The basil EGS and petunia IGS are closely related to a number of other NADPH-dependent enzymes that act on phenylpropanoid-derived substrates. Structurally, the PIP-family proteins organize around an N-terminal, Rossman-fold domain, containing a core, six-stranded parallel β-sheet flanked on each face by an α-helical layer. In summary, a mechanistic scheme emerges in which binding of the coniferyl acetate substrate within the active site of EGS leads to deprotonation of the p-hydroxy group (PUSH) coupled with expulsion of acetate ion from the C1 substituent (PULL).

The monoclinic structure also contains two EGS/NADP+ complexes per asymmetric unit and was refined at 1.6-Å resolution resulting in crystallographic R-factors of 0.210 and 0.229. Intruigingly, in the monoclinic structure of unliganded EGS-NADP+, a nitrate anion from the crystallization medium occupies the site of the bridging water molecule, and may mimic the hydroxide ion that develops during the catalytic reaction. The structures of EGS complexed with NADP+ or NADPH provide the first structural characterization of nicotinamide-cofactor binding by the PIP family of enzymes (previous crystallographic analyses had yielded only apo-enzyme structures). The cofactor is bound through a large number of polar and non-polar interactions. The nicotinamide ring adopts the anti conformation with its B-face stacked against the side chain of Phe154 and its A-face directed towards the substrate-binding pocket. In contrast, the anti-conformer of the nicotinamide ring observed in EGS is consistent with the class-A reductase (donation of the pro-R hydride) activity of the PIP-family enzymes. Detailed inspection of the hydrogen-bonding network involving the ε-amino group of Lys132 suggests that this group exists formally in the unprotonated–NH2 state and is the donor in hydrogen-bond interactions with the 2′-hydroxyl group of the nicotinamide-ribose and the backbone carbonyl oxygen of residue 110. With an available lone pair of electrons, the amino group can serve as the acceptor in a hydrogen bond with the bridging water molecule, and most importantly, thereby act as a general base.

>MEENGMKSKILIFGGTGYIGNHMVKGSLKLGHPTYVFTRPNSSKTTLLDEFQSLGAIIVKGELDEHEKLVELMKKVDVVISALAFPQILDQFKILEAIKVAGNIKRFLPSDFGVEEDRINALPPFEALIERKRMIRRAIEEANIPYTYVSANCFASYFINYLLRPYDPKDEITVYGTGEAKFAMNYEQDIGLYTIKVATDPRALNRVVIYRPSTNIITQLELISRWEKKIGKKFKKIHVPEEEIVALTKELPEPENIPIAILHCLFIDGATMSYDFKENDVEASTLYPELKFTTIDELLDIFVHDPPPPASAAF[2x]meropenem, bound form | C17 H27 N3 O5 S | 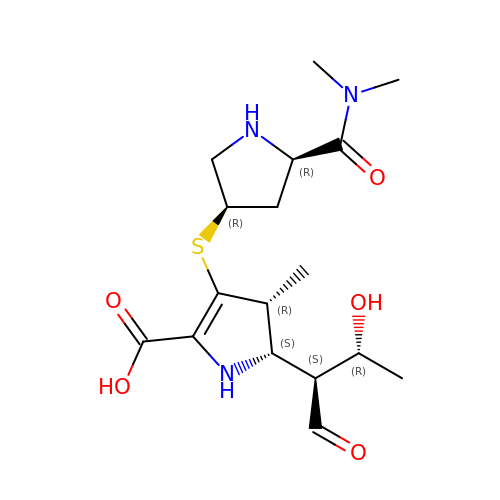DYQHXZPAIVAJRU-PCEBWVJKSA-N>MEGGGKPNSSSNSRDDGNSVFPAKASATGAGPAAAEKRLGTPPGGGGAGAKEHGNSVCFKVDGGGGGGGGGGGGEEPAGGFEDAEGPRRQYGFMQRQFTSMLQPGVNKFSLRMFGSQKAVEKEQERVKTAGFWIIHPYSDFRFYWDLIMLIMMVGNLVIIPVGITFFTEQTTTPWIIFNVASDTVFLLDLIMNFRTGTVNEDSSEIILDPKVIKMNYLKSWFVVDFISSIPVDYIFLIVEKGMDSEVYKTARALRIVRFTKILSLLRLLRLSRLIRYIHQWEEIFHMTYDLASAVVRIFNLIGMMLLLCHWDGCLQFLVPLLQDFPPDCWVSLNEMVNDSWGKQYSYALFKAMSHMLCIGYGAQAPVSMSDLWITMLSMIVGATCYAMFVGHATALIQSLDSSRRQYQEKYKQVEQYMSFHKLPADMRQKIHDYYEHRYQGKIFDEENILNELNDPLREEIVNFNCRKLVATMPLFANADPNFVTAMLSKLRFEVFQPGDYIIREGAVGKKMYFIQHGVAGVITKSSKEMKLTDGSYFGEICLLTKGRRTASVRADTYCRLYSLSVDNFNEVLEEYPMMRRAFETVAIDRLDRIGKKNSILLQKFQKDLNTGVFNNQENEILKQIVKHDREMVQAIAPINYPQMTTLNSTSSTTTPTSRMRTQSPPVYTATSLSHSNLHSPSPSTQTPQPSAILSPCSYTTAVCSPPVQSPLAARTFHYASPTASQLSLMQQQPQQQVQQSQPPQTQPQQPSPQPQTPGSSTPKNEVHKSTQALHNTNLTREVRPLSASQPSLPHEVSTLISRPHPTVGESLASIPQPVTAVPGTGLQAGGRSTVPQRVTLFRQMSSGAIPPNRGVPPAPPPPAAALPRESSSVLNTDPDAEKPRFASNL[4x]

The hyperpolarization-activated cyclic nucleotide-gated (HCN) channels play a crucial role in regulating neuronal excitability. The HCN1 subtype is notably distinguished by its primary localization in both the central and peripheral nervous systems. Overall, the structures form a symmetric homotetramer, each subunit comprises six alpha-helical transmembrane domains, with two forming the pore (S5-S6) and four forming the voltage sensor domain (S1-S4). The cytoplasmic domain contains an N-terminal conserved HCN domain (HCND) and a C-terminal cyclic nucleotide-binding domain, which is connected to transmembrane helix S6 through a helical C-linker domain.

Here, we present the cryo-electron microscopy structure of human HCN1 channel in complex with inhibitor ivabradine, the drug on the market that acts on HCN channels. Reconstructions of HCN1 in the ivabradine bound states were carried out to an overall resolution of 3.23 Å. The overall architecture of ivabradine-bound HCN1 closely resembles the previously characterized apo state, with an RMSD of 0.5 Å. A nonprotein density is observed, surrounded by the S1, S4, and the unique HCND at the interface between the lipid bilayer and cytoplasmic side, a feature not present in any of the previous HCN1 and HCN4 structures. Specifically, the side chain of F143 on S1 forms π-stacking interactions with the methoxyphenyl ring of ivabradine. Additionally, N107 and F109 on the HCND, D140 on S1, W281, F285, and Y289 on S4 exhibit hydrophobic and van der Waals interactions with ivabradine. Notably, mutations such as D140A and F143A led to a dramatic decrease in ivabradine potency. In the ivabradine binding site, the residues F143, W281, and F285 exhibit slight inward conformational changes compared to apo HCN1, likely induced by ivabradine binding. In the ivabradine-bound state, W281 is oriented toward S1, nestled within a hydrophobic cavity at the interface of S4, S1, and the HCND. The inhibitor acts like a wedge, engendering hydrophobic interactions with W281, thus preventing the conformational change of the S4 helix and maintaining the HCN1 channel in a closed conformation.>[2x]ASRDPQGRPDSPRERTPKGKPHAQQPGRASASDSSAPWSRSTDGTILAQKLAEEVPMDVASYLYTGDSHQLKRANCSGRYELAGLPGKWPALASAHPSLHRALDTLTHATNFLNVMLQSNKSREQNLQDDLDWYQALVWSLLEGEPSISRAAITFSTDSLSAPAPQVFLQATREESRILLQDLSSSAPHLANATLETEWFHGLRRKWRPHLHRRGPNQGPRGLGHSWRRKDGLGGDKSHFKWSPPYLECENGSYKPGWLVTLSSAIYGLQPN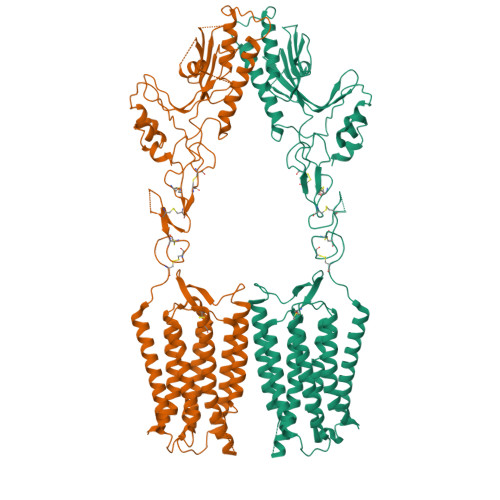LVPEFRGVMKVDINLQKVDIDQCSSDGWFSGTHKCHLNNSECMPIKGLGFVLGAYECICKAGFYHPGVLPVNNFRRRGPDQHISGSTKDVSEEAYVCLPCREGCPFCADDSPCFVQEDKYLRLAIISFQALCMLLDFVSMLVVYHFRKAKSIRASGLILLETILFGSLLLYFPVVILYFEPSTFRCILLRWARLLGFATVYGTVTLKLHRVLKVFLSRTAQRIPYMTGGRVMRMLAVILLVVFWFLIGWTSSVCQNLEKQISLIGQGKTSDHLIFNMCLIDRWDYMTAVAEFLFLLWGVYLCYAVRTVPSAFHEPRYMAVAVHNELIISAIFHTIRFVLASRLQSDWMLMLYFAHTHLTVTVTIGLLLIPKFSHSSNNPRDDIATEAYEDELDMGRSGSYLNSSINSAWSEHSLD(4~{R})-4-[3-[(4-azanyl-2-methyl-pyrimidin-5-yl)methyl]-4-methyl-5-[2-[oxidanyl(phosphonooxy)phosphoryl]oxyethyl]-1,3-thiazol-3-ium-2-yl]-4-oxidanyl-butanoic 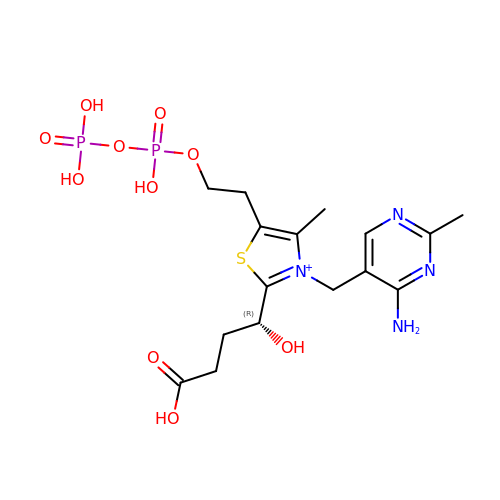acid | C16 H25 N4 O10 P2 S | ZWUKRGPVMMTMAF-GFCCVEGCSA-O> MRIGEWMRGLLLCAGLMMCGVVHADISTVPDETYDALKLDRGKATPKETYEALVKRYKDPAHGAGKGTMGDYWEPIAISIYMDPNTFYKPPVSPKEVAERKDCVECHSDETPVWVRAWKRSTHANLDKIRNLKSDDPLYYKKGKLEEVENNLRSMGKLGEKETLKEVGC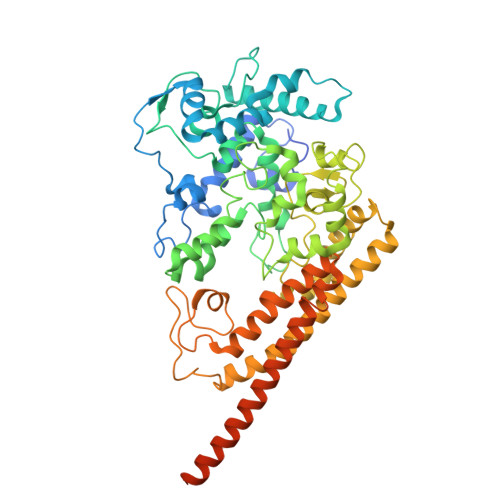IDCHVDVNKKDKADHTKDIRMPTADTCGTCHLREFAERESERDTMVWPNGQWPAGRPSHALDYTANIETTVWAAMPQREVAEGCTMCHTNQNKCDNCHTRHEFSAAESRKPEACATCHSGVDHNNWEAYTMSKHGKLAEMNRDKWNWEVRLKDAFSKGGQNAPTCAACHMEYEGEYTHNITRKTRWANYPFVPGIAENITSDWSEARLDSWVLTCTQCHSERFARSYLDLMDKGTLEGLAKYQEANAIVHKMYEDGTLTGQKTNRPNPPEPEKPGFGIFTQLFWSKGNNPASLELKVLEMAENNLAKMHVGLAHVNPGGWTYTEGWGPMNRAYVEIQDEYTKMQELSALQARVNKLEGKQTSLLDLKGTGEKISLGGLGGGMLLAGALALIGWRKRKQTRA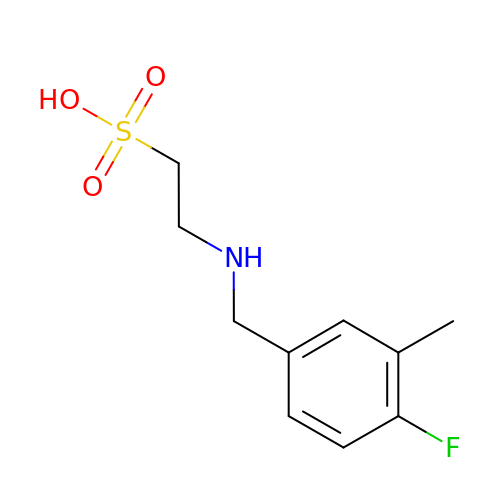2-[(4-fluoro-3-methylbenzyl)amino]ethanesulfonic acid | C10 H14 F N O3 S | FDPJRTHZQIQRJH-UHFFFAOYSA-N> MLTPTPD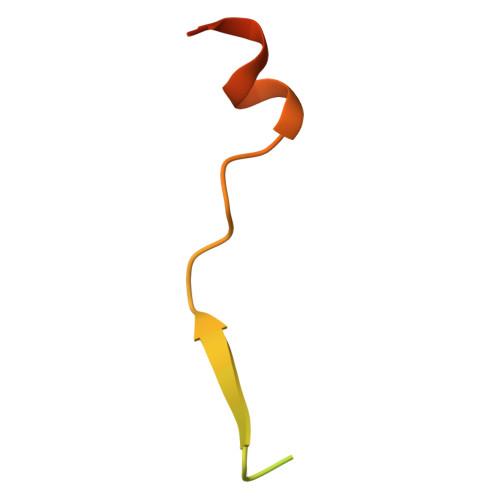SSPRSTSSPSQSKNGSFTPRTANILKPLMSPPSREEIMATLLDHD>AMSKKEININNYNDDAIQVLEGLDAVRKRPGMYIGSTDGAGLHHLVWEIVDNAVDEALSGFGDRIDVTINKDGSLTVQDHGRGMPTGMHAMGIPTVEVIFTILHAGGKFGQGGYKTSGGLHGVGSSVVNALSSWLEVEITRDGAVYKQRFENGGKPVTTLKKIGTAPKSKTGTKVTFMPDATIFSTTDFKYNTISERLNESAFLLKNVTLSLTDKRTDEAIEFHYENGVQDFVSYLNEDKEILTPVLYFEGEDNGFQVEVALQYNDGFSDNILS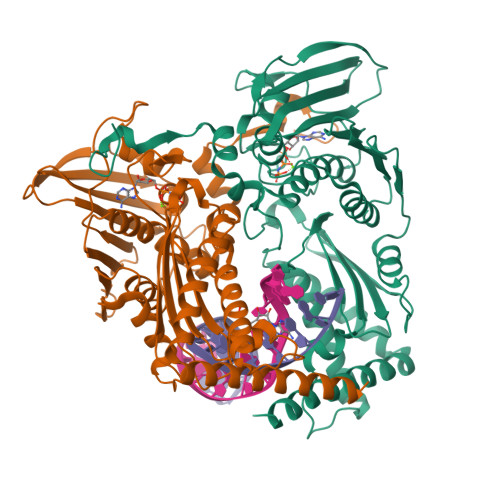FVNNVRTKDGGTHETGLKSAITKVMNDYARKTGLLKEKDKNLEGSDYREGLAAVLSILVPEEHLQFEGQTKDKLGSPLARPVVDGIVADKLTFFLMENGELASNLIRKAIKARDAREAARKARDESRNGHHHHHH[4x]> LENKNATVEQTKENIFLVPLKHLRDSQFVGELLVGTPPQTVYPIFDTGSTNVWVVTTACEEESCKKVRRYDPNKSKTFRRSFIEKNLHIVFGSGSISGSVGTDTFMLGKHLVRNQTFGLVESESNNNKNGGDNIFDYISFEGIVGLGFPGMLSAGNIPFFDNLLKQNPNVDPQFSFYISPYDGKSTLIIGGISKSFYEGDIYMLPVLKESY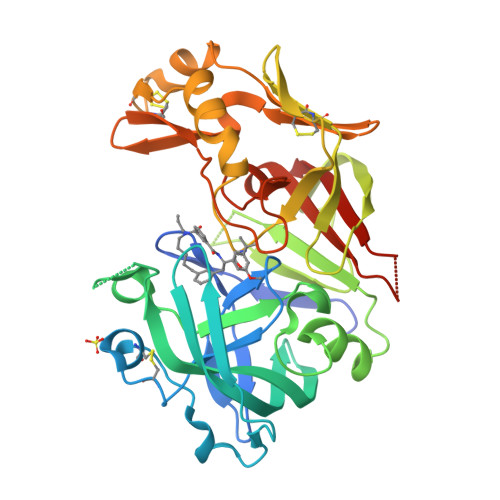WEVKLDELYIGKERICCDEESYVIFDTGTSYNTMPSSQMKTFLNLIHSTACTEQNYKDILKSYPIIKYVFGELIIELHPEEYMILNDDVCMPAYMQIDVPSERNHAYLLGSLSFMRNFFTVFVRGTESRPSMVGVARAKSKNEPEA> PVNPCCYYPCQHQGICVRFGLDRYQCDCTRTGYSGPNCTIPEIWTWLRTTLRPSPSFIHFLLTHGRWLWDFVNATFIRDTLMRLVLTVRSNLIPSPPTYNIAHDYISWESFSNVSYYTRILPSVPRDCPTPMGTKGKKQLPDAEFLSRRFLLRRKFIPDPQGTNLMFAFFAQHFTHQFFKTSGKMGPGFTKALGHGVDLGHIYGDNLERQYQLRLFKDGKLKYQMLNGEVYPPSVEEAPVLMHYPRGIPPQSQMAVGQEVFGLLPGLMLYATIWLREHNRVCDLLKAEHPTWGDEQLFQTARLILIGETIKIVIEEYVQQLSGYFLQLKFDPELLFGAQFQYRNRIAMEFNQLYHWHPLMPDSFRVGPQDYSYEQFLFNTSMLVDYGV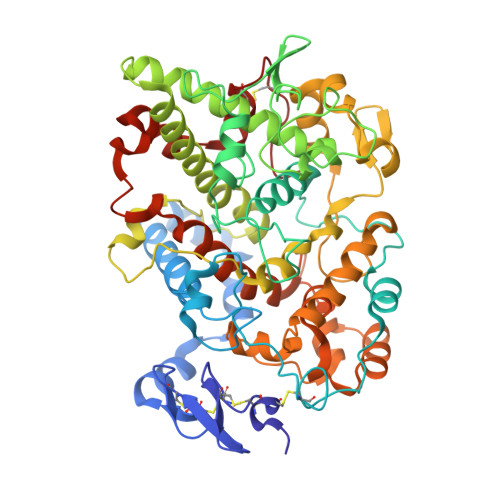EALVDAFSRQPAGRIGGGRNIDHHILHVAVDVIKESRVLRLQPFNEYRKRFGMKPYTSFQELTGEKEMAAELEELYGDIDALEFYPGLLLEKCHPNSIFGESMIEMGAPFSLKGLLGNPICSPEYWKASTFGGEVGFNLVKTATLKKLVCLNTKTCPYVSFHVPD>[3x]SVRSSSRTPSDK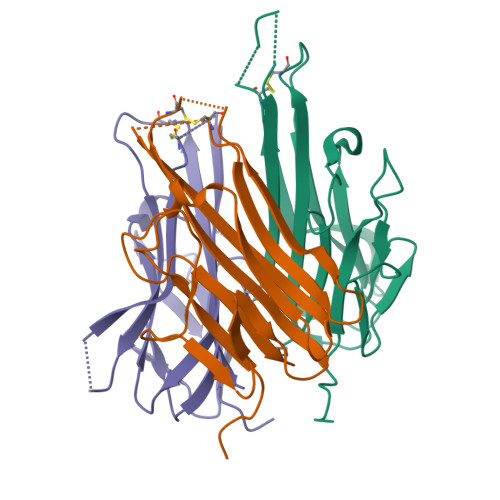PVAHVVANPQAEGQLQWLNRRANALLANGVELRDNQLVVPSEGLYLIYSQVLFKGQGCPSTHVLLTHTISRIAVSYQTKVNLLSAIKSPCQRETPEGAEAKPWYEPIYLGGVFQLEKGDRLSAEINRPDYLDFAESGQVYFGIIAL2-{[4-amino-3-(3-hydroxyprop-1-yn-1-yl)-1H-pyrazolo[3,4-d]pyrimidin-1-yl]methyl}-5-methyl-3-(2-methylphenyl)quinazolin-4(3H)-one 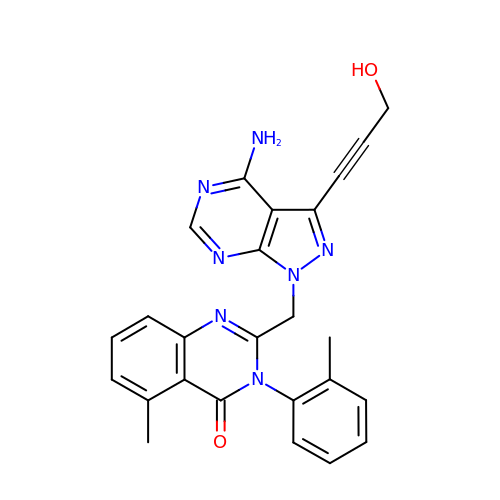| C25 H21 N7 O2 | GJBJSDBBRWPDBE-UHFFFAOYSA-N(1R,2S,3S,4R,6S)-4,6-diamino-3-{[3-deoxy-4-C-methyl-3-(methylamino)-beta-L-arabinopyranosyl]oxy}-2-hydroxycyclohexyl 2-amino-2,3,4,6-tetradeoxy-6-[({3-hydroxy-2-methyl-5-[(phosphonooxy)methyl]pyridin-4-yl}methyl)amino]-alpha-D-erythro-hexopyranoside 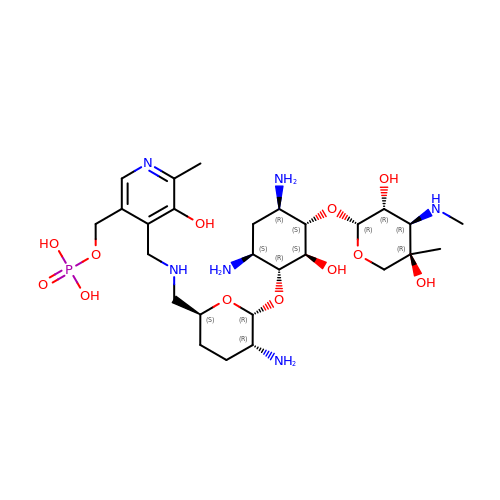| C27 H49 N6 O12 P | RIDGEVUBNCTQEZ-IXQBVWJDSA-N The RNA-binding motif protein RBM5 belongs to a family of multi-domain RNA binding proteins that regulate alternative splicing of genes important for apoptosis and cell proliferation and have been implicated in cancer. RBM5 comprises multiple domains, including an arginine/serine rich (RS) region, two RNA recognition motif (RRM) domains (RRM1 and RRM2), two zinc finger domains (ZnF1 and ZnF2), an OCRE domain (OCtamer REpeat)32 and a glycine-rich domain (G-patch) at the C-terminus. Notably, both of the RBM5 RRM domains are non-canonical as they lack the consensus aromatic residue in RNP2, which might impact their RNA recognition. To study how RBM5 recognizes cis-regulatory RNA motifs, we investigated the roles of the three RNA binding domains (RRM1-ZnF1-RRM2), which are connected by linkers L0 (7 residues, between RRM1 and ZnF1) and L1 (20 residues, between ZnF1 and RRM2).

Crystals of RRM1-ZnF1S bound to GGCU_10 RNA (lacking two bases at the 3′-end of GGCU_12) diffracted to an overall resolution of 3.5 Å. The structure was solved with molecular replacement using the RBM5 RRM1-ZnF1 apo structure and showed interpretable electron density for seven RNA nucleotides (UGGCUCU). The RNA is sandwiched between the RRM1 and ZnF1 tandem domains and is recognized via a network of hydrophobic and polar interactions. The first uracil (U1) base forms hydrogen bonds with Arg140 from RRM1 and N2 of guanine at position 2 (G2). G2 further stacks with Met101 and RNP1 aromatic residue Phe142 of RRM1. G3 is involved in an intricate set of specific interactions spanning both RRM1 and ZnF1. It stacks with Phe202 of ZnF1 and backbone of Lys133, Met132 of RRM1, while its phosphate backbone is recognized by polar interactions with Asn194 and Arg198 of ZnF1. Arg203 in ZnF1 forms hydrophobic contacts with C4 and Asp128 from the RRM1 establishes hydrogen bonds with the riboses of both C4 and U5. U5 and C6 are solvent exposed and not involved in any base-specific interactions. In summary, the specific recognition of the RNA core (U1-G2-G3) involves a hydrophobic groove between RRM1 and ZnF1 (Phe142, Met101, Met132, and Phe202) and important electrostatic interactions involving residues from both domains (Arg140, Asn194, and Arg198). In our structure however, no hydrophobic interactions are observed between the RNA and the aromatic residue at position 5 of RNP1 while position 3 of RNP1 (Phe142) and position 2 of RNP2 (Met101) stack with G2 of RNA in a non-canonical way.

>[4x]MGERESKTIMLRGLPTTITESDIREMMESFEGPQPADVRLMKRKTGVSRGFAFVEFYHLQDATSWMEANQKKLVIQGKHIAMHYSNPRPKFEDWLCNKCGLNNFRKRLKCFRCGADKFD pyridine-4-carboxylic acid | C6 H5 N O2 | 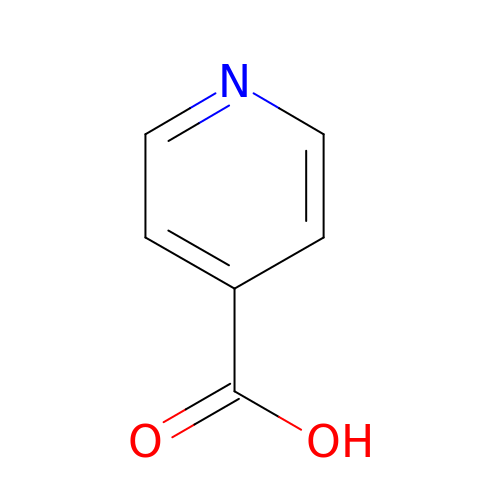TWBYWOBDOCUKOW-UHFFFAOYSA-N> HHHHHHMSGENLYFQGASAAIVTDTGGVDDKSFNQSAWEGLQAWGK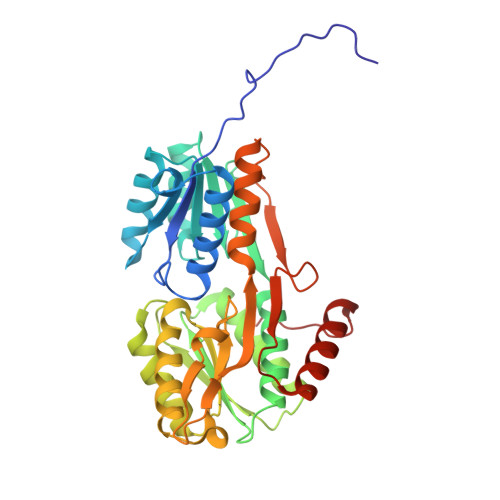EHNLSKDNGFTYFQSTSEADYANNLQQAAGSYNLIFGVGFALNNAVKDAAKEHTDLNYVLIDDVIKDQKNVASVTFADNESGYLAGVAAAKTTKTKQVGFVGGIESEVISRFEAGFKAGVASVDPSIKVQVDYAGSFGDAAKGKTIAAAQYAAGADIVYQVAGGTGAGVFAEAKSLNESRPENEKVWVIGVDRDQEAEGKYTSKDGKESNFVLVSTLKQVGTTVKDISNKAERGEFPGGQVIVYSLKDKGVDLAVTNLSEEGKKAVEDAKAKILDGSVKVPEK> MNSEYDY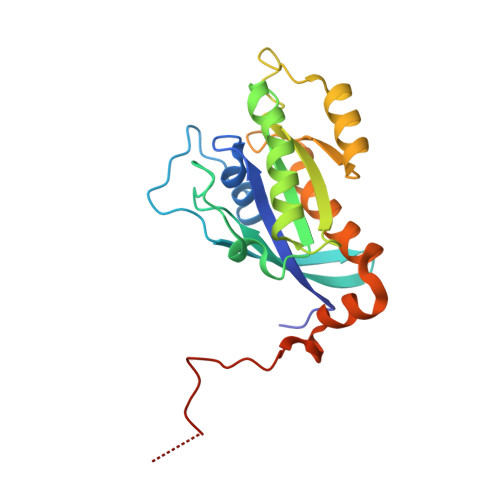LFKLLLIGNSGVGKSCLLLRFSDDTYTNDYISTIGVDFKIKTVELDGKTVKLQIWDTAGQERFRTITSSYYRGSHGIIIVYDVTDQESFNGVKMWLQEIDRYATSTVLKLLVGNKCDLKDKRVVEYDVAKEFADANKMPFLETSALDSTNVEDAFLTMARQIKESMSQQNLNETTQKKEDKGNVNLKGQSLTNTGGGCC>[2x]MKRIFEVQPWNVITHTFDPKDKRLQESMTSLGNGYMGMRGDFEEGYSGDSLQGIYLGGVWYPDKTRVGWWKNGYPKYFGKVVNAVNFIKLPIEINGEPVDLAKDKISDFTLDLDMHQGVLNRSFVVERGAVRVALNFQRFLSVAQPELSVQKVTVKNLSDAEVDVTLKPSIDADVMNEEANYDERFWDVLATDQQADRGSIVAKTTPNPFGTPRFTSGMEMRLVTDLKNVAITQPNEKEVTTAYTGKLAPQASAELEKRVIVVTSRDYDTQESLTAAMHQLSDKVAQSSYEDLLNAHTAIWAQRWEKSDVVIKGDDESQQGIRFNLFQLFSTYYGEDARLNIGPKGFTGEKYGGATYWDTEAFAFP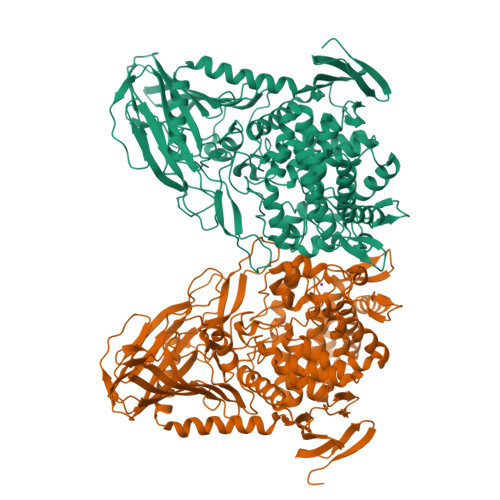VYLGITDPKVTRNLLMYRYKQLDGAYINAQEQGLKGALFPMVTFDGIECHNEWEITFEEIHRNGDIAFAIYNYTRYTGDDSYVLHEGAKVLTEISRFWADRVHFSKRNNQYMIHGVTGADEYENNVDNNWDTNMLAQWTLKYTLEILGKVDQDTAKQLDVSDEEKTKWQDIVDRMYLPYDKDLNIFVQHDGFLDKDIEPVSSIPADQRPINQNWSWDKILRSPYIKQGDVLQGIWDFIDDYTPEQKKANFDFYEPLTVHESSLSPAIHSVLAADLHYEDKAVELYSRTARLDLDNYNNDTTDGLHITSMTGAWIAVVQGFAGMRVRDGQLHYAPFLPKTWTSYTFRQVFRDRLIEVSVHADGPHFKLLSGEPLTIDVAGAAAAAAAAA>GSVDDSAQSDLKEVMVLNATESFVYEPKEQKKMFHATVATENEVFRVKVFNIDLKEKFTPKKIIAIANYVCRNGFLEVYPFTLVADVNADRNMEIPKGLIRSASVTPKINQLCSQTKGSFVNGVFEVHKKNVRGEFT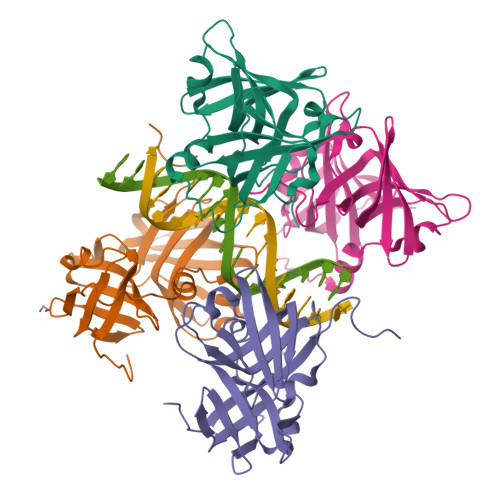YYEIQDNTGKMEVVVHGRLTTINCEEGDKLKLTCFELAPKSGNTGELRSVIHSHIKVIKTRKNAAAS[4x]> GNDQSLRSSLLGLRQLLRELPGDEAPLDALAETVLALLAQYGSLRIAGLYRVRYDRTPEPQPLATLGEMPALDADDLLVRTCLERGELVSVRQELLERGEQRAHSALQVCVPLVDTDGRILALLAVEQMPFFVFNERTFSLLAILAGHIADLLQSDRRALQLADIDAQRFSQYLKRSLLDARDHGLP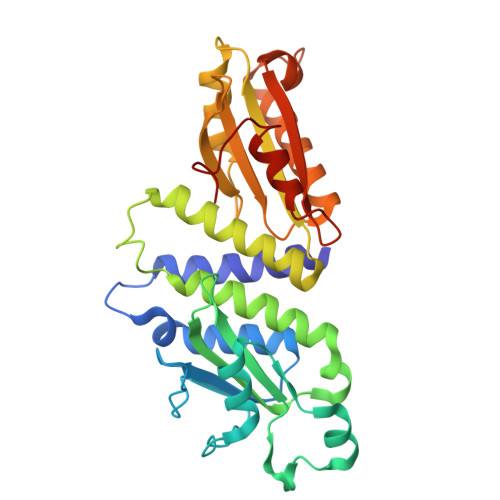ACLYAFELTDARYGEEVQRLLEGSQRGLDVQLRLRNDEGRRVLLVLLPLTSAEGSQGYLQRLRILFAERFGQARELESLGVRIRQYELDAGNDRQALGHFLFNECGLNDQQVA> MWSHPQFEKENLYFQGPDYLPVDRYLPVDRYLPHEAPMVLLEQVINVSDNHVHCQVTVSRDGVLSPFLNQDGHLPGWFAIEMMAQAIGVWSGWHRKERKEADSALGMLLGGRAVRCQVPAFTQG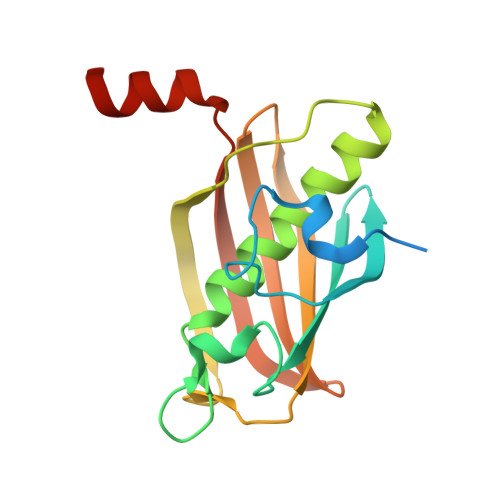SVLDIQMNLLLQDEKFGSFEGEISCYGTVLVTGRLNTYQPNKTELIQLINKQDGVA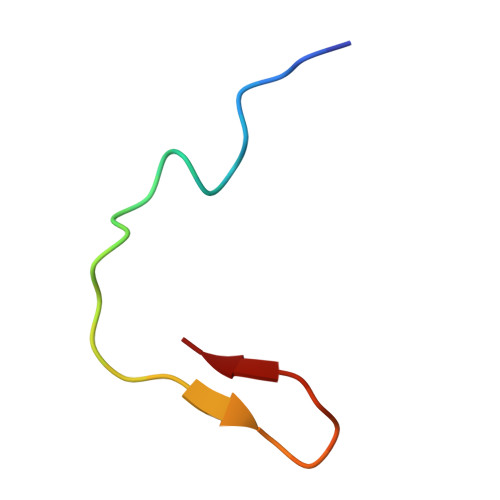> DENLPEWAIENPSKLGGSFDASGAFHG> GSSGSSGDGTCTGAMPDGALDTAVCADEVGSEEDLYDDLHSSSHHYSHPGGGGEQLAINELISDGSVVCAEALWDHVTMDDQELGFKAGDVIEVMDATNREWWWGRVADGEGWFPASFVRLRVNQDEPADDDAPLAGNSGAEDGGAEAQSSKDQMRTNVINEILSTERDYIKHLRDICEGYVRQCRKRADMFSEEQLRTIFGNIEDIYRCQKAFVKALEQRFNRERPHLSELGACFLEHQADFQIYSEYCNNHPNACVELSRLTKLSKYVYFFEACRLLQKMIDISLDGFLLTPVQKICKYPLQ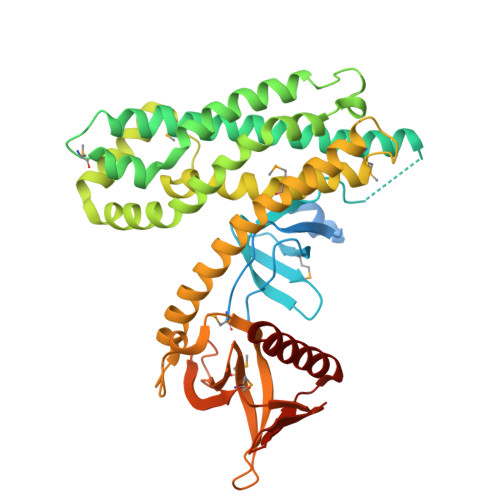LAELLKYTHPQHRDFKDVEAALHAMKNVAQLINERKRRLENIDKIAQWQSSIEDWEGEDLLVRSSELIYSGELTRVTQPQAKSQQRMFFLFDHQLIYCKKDLLRRDVLYYKGRLDMDGLEVVDLEDGKDRDLHVSIKNAFRLHRGATGDSHLLCTRKPEQKQRWLKAFAREREQVQLD> MSLLSADEKITESLRSTLSDVLPDQLQTYIRTVLQFSGRPEGANLLTGPNTEIEFFSQDPNKNFPNIFAKYSNVLTVSSDPNFITSEDEEVKIIWGRHGSDSLIGFDPGADLVGKRRIDIFLGDFIDEQFNPIPGALNAGKSWSDRFILGDWQKPYYFEDDETLGLNQSAMILDFNPNEDVIQLHGDRQDYELVNISLGTAIFWREKKGYDLIGVLGGVSDLSLKGDYFEFKGNTAPKTVLKTAEHIGTAANDYIFSSTVDAKGNFYVGGGTGGSLGGRNIGARDAWLAKYDSNGNQRWSRQFGSTGTESLWGMASDGSNIYVAGNTTGQLENNTVKGGNDAYLAKYDSDGNQVWIKQNGTYTLEESYKITVDSSGNIYTAGHTFGSLGGPNQNLEQGEVFELPSTDGYVAKFDSNGNQLWVAQFGTITLDDNWGVAADNNGNVFAGGNTKGSFGA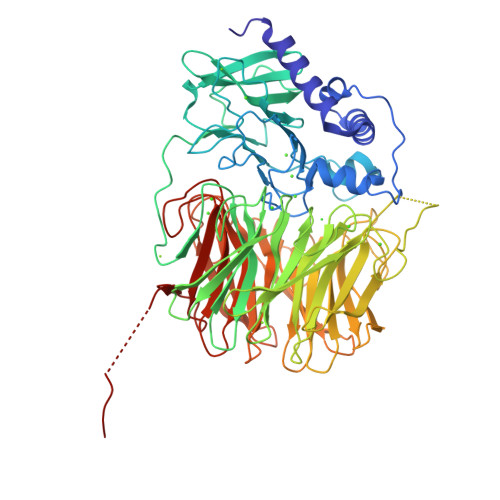KNTGTAGEYDAWLVKLNKDGQTDWVRQFGTPNYDFMWDIETDSLGDIYATGWTLGDLGGKNAGSYDVWLAKYNTNGNQLWIKQFGTSEDDAPFLDGIDIDANDNIFLTGNTNGNLGGANAGSYDAWAAKFDKDGNQLWLKQFGTPDYDTATTVTAVNFGKLYVSGITEGSLGTTNAGSYDSWALKLDADNGEIQDFNSSTNTFGQTGFLNL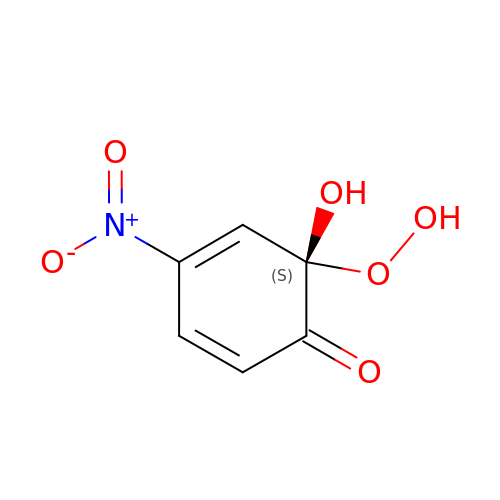(1S)-1-HYDROPEROXY-1-HYDROXY-2-KETO-5-NITROCYCLOHEXA-3,5-DIENE | C6 H5 N O6 | FWUJUIQFDWUIAR-LURJTMIESA-N NALPHA-[(TRANS-4-METHYLCYCLOHEXYL)CARBONYL]-N-PYRIDIN-4-YL-D-TRYPTOPHANAMIDE | C24 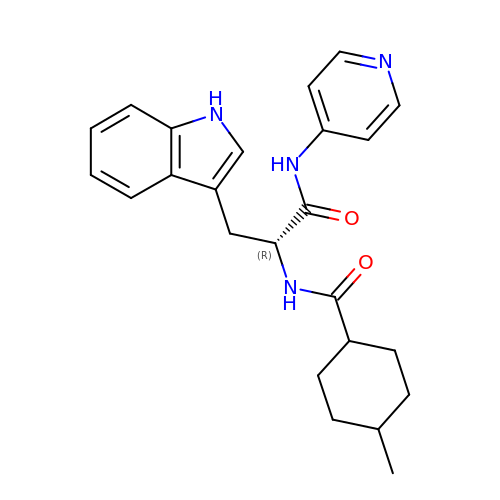H28 N4 O2 | ICFUCABJWQGTGU-DRSNIGMVSA-N> TSSATSSSSMILKYPYRVVDTHEKLKEAVTSLQGARSIALDIEAFCTTDQAKQLGRISLVQACSDAKPVVFLFDVLTLTPDVFVKDMQSLLSDREIRKLFFDCRRDVEALSCQLGVKPEGVLDLQVFFTAIQWKLRSVNRRSGMGYVLKSVAGLTRQEGDSAVQTAMTLGNRPVWDIRPLPDHFLEYAAGDVRHILLLSNYLVGNKDVPVDVVAVERLTAQYVEHYAVGKPVITEADA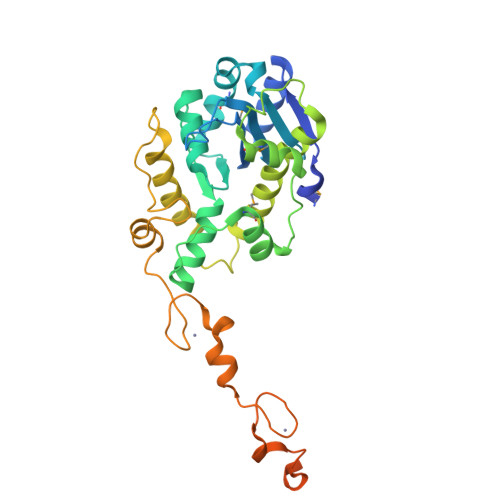TPAEVNRAWLERYIGPGGGCHFCGAKGHTEAECFKKQNGKAKCSFCGEVGHTARNCFKKHPQLLTCEKCGQLGHTGTSCFRTNPCKHCGGPHSSANCHKVIWQQKRLGENSLH>[2x]GPMRSRIFKIIVIGDSNVGKTCLTYRFCAGRFPDRTEATIGVDFRERAVEIDGERIKIQLWDTAGQERFRKSMVQHYYRNVHAVVFVYDMTNMASFHSLPSWIEECKQHLLAND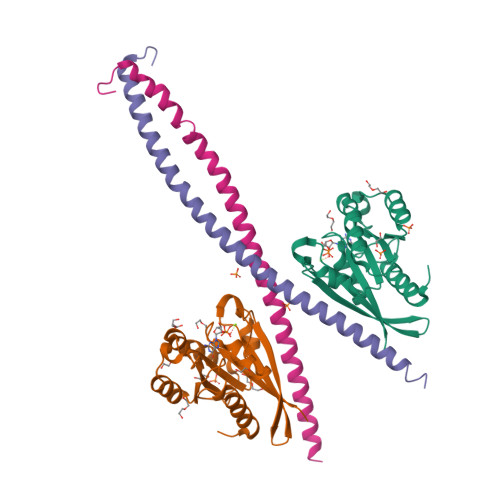IPRILVGNKCDLRSAIQVPTDLAQKFADTHSMPLFETSAKNPNDNDHVEAIFMTLAHKLKSHKPLMLSQPPDNGIILK;>MLETNCLDLRTKLQDLEVANQTLKDEYDALQITFTALEEKLRKTTEENQELVTRWMAEKAQEANRLNAENEKDSRRRQARLQKELAEAAKEPLPVEQDDDIEVIVDETSDHTEETSPVRAVSRAAT[2x]> MGTQLESTFEQDVSQMEHDMADQEEHDLSSFERKKLPTDFDPSLYDISFQQIDAEQSVLNGIKDENTSTVVRFFGVTSEGHSVLCNVTGFKNYLYVPAPNSSDANDQEQINKFVHYLNETFDHAIDSIEVVSKQSIWGYSGDTKLPFWKIYVTYPHMVNKLRTAFERGHLSFNSWFSNGTTTYDNIAYTLRLMVDCGIVGMSWITLPKGKYSMIEPNNRVSSCQLEVSINYRNLIAHPAEGDWSHTAPLRIMSFDIECAGRIGV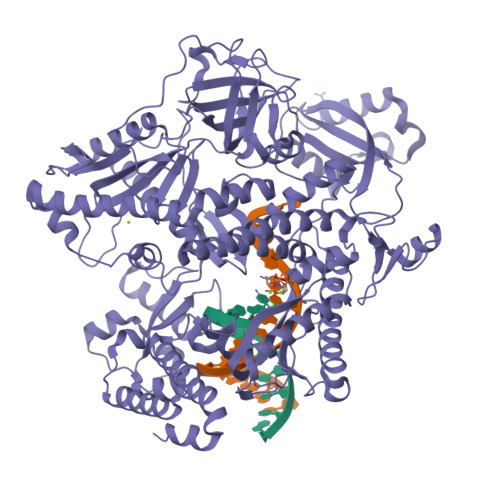FPEPEYDPVIQIANVVSIAGAKKPFIRNVFTLNTCSPITGSMIFSHATEEEMLSNWRNFIIKVDPDVIIGYNTTNFDIPYLLNRAKALKVNDFPYFGRLKTVKQEIKESVFSSKAYGTRETKNVNIDGRLQLDLLQFIQREYKLRSYTLNAVSAHFLGEQKEDVHYSIISDLQNGDSETRRRLAVYCLKDAYLPLRLMEKLMALVNYTEMARVTGVPFSYLLARGQQIKVVSQLFRKCLEIDTVIPNMQSQASDDQYEGATVIEPIRGYYDVPIATLDFNSLYPSIMMAHNLCYTTLCNKATVERLNLKIDEDYVITPNGDYFVTTKRRRGILPIILDELISARKRAKKDLRDEKDPFKRDVLNGRQLALKISANSVYGFTGATVGKLPCLAISSSVTAYGRTMILKTKTAVQEKYCIKNGYKHDAVVVYGDTDSVMVKFGTTDLKEAMDLGTEAAKYVSTLFKHPINLEFEKAYFPYLLINKKRYAGLFWTNPDKFDKLDQKGLASVRRDSCSLVSIVMNKVLKKILIERNVDGALAFVRETINDILHNRVDISKLIISKTLAPNYTNPQPHAVLAERMKRREGVGPNVGDRVDYVIIGGNDKLYNRAEDPLFVLENNIQVDSRYYLTNQLQNPIISIVAPIIGDKQANGMFVV>MGPILSKNEILEETVPELPEDYEISEKTIITPIGVLKSAFENNIIIHATMSGEKRVLKEGSIFCLEDRTLIGMLTEVFGPLQNPFYRIKLPDSKKNL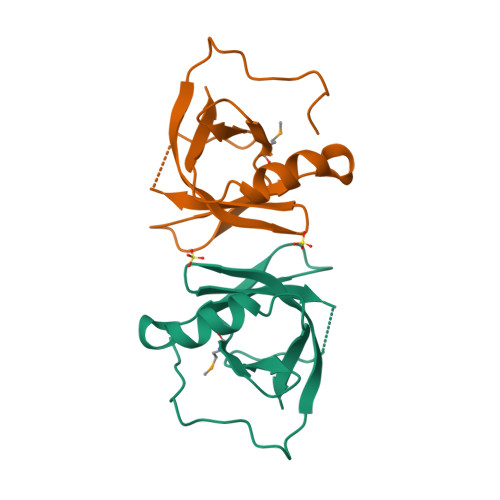FDELKVRLGEKAFIVTPDAHWIDTFELKHHHHHH[6x]> QEITVDEFSNIRENPVTPNNPEPSAPVIDPTAYIDPQASVIGEVTIGANVMVSPMASIRSDEGMPIFVGDRSNVQDGVVLHALETINEEGEPIEDNIVEVDGKEYAVYIGNNVSLAHQSQVHGPAAVGDDTFIGMQAFVFKSKVGNNCVLEPRSAAIGVTIPDGRYIPAGMVVTS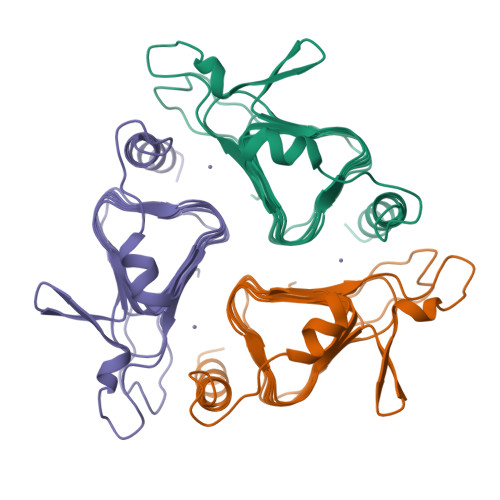QAEADKLPEVTDDYAYSHTNEAVVYVNVHLAEGYKETS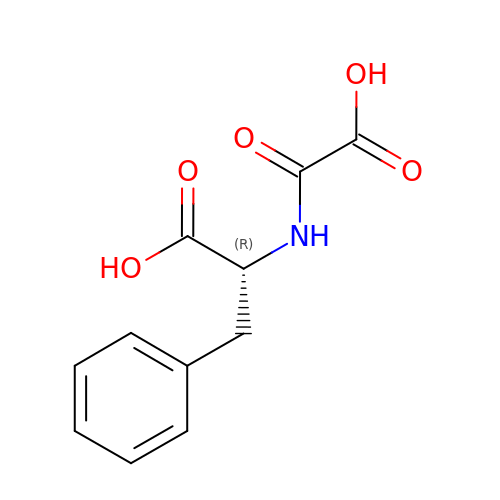N-(CARBOXYCARBONYL)-D-PHENYLALANINE | C11 H11 N O5 | ULQWGBCNOHBNDB-MRVPVSSYSA-N> NLDNKLDGFYIAPAFMDKLVVHITKNFLKLPNIKVPLILGIWGGKGQGKSFQCELVFRKMGINPIMMSAGELESGNAGEPAKLIRQRYREAAEIIRKGNMCCLFINDLDAGAGRMGGTTQYTVNNQMVNATLMNIADNPTNVQLPGMYNKQENARVPIIVTGNDFSTLYA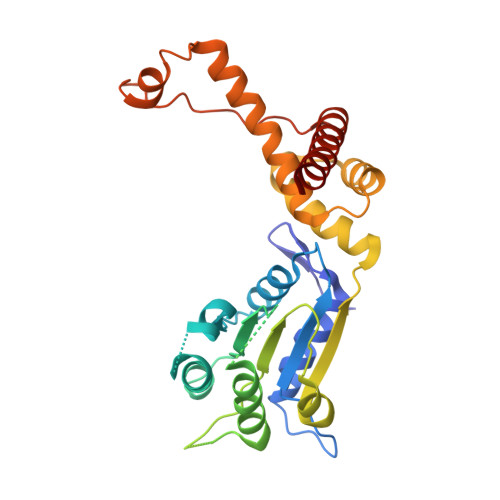PLIRDGRMEKFYWAPTREDRIGVCTGIFRTDNVPAEDVVKIVDNFPGQSIDFFGALRARVYDDEVRKWVSGTGIEKIGDKLLNSFDGPPTFEQPKMTIEKLLEYGNMLVQEQENVKRVQLADK>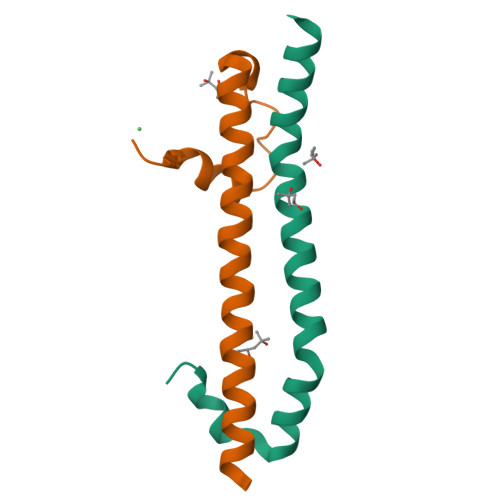 GEFEFLKFLTFDDLNQRLCNIDHEMELEIEQLNKKYNAKRQPIVDAMNAKRKRQQNI;> LLEEIPKWLAVYSEADSSKDHLLQFNMFSLPELEGFDSMLVRLFKQELGTIVGFYERYRRALILEKNRRA> GAMAMNEFTQISGYVNAFGSQRGSVLTVKVENDEGWTLVEEDFDRADYGSDPEFVAEV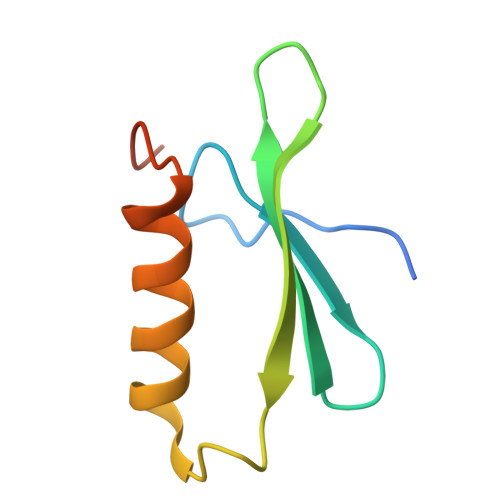SSYLKRNGGIKDLTKVLTR GMP synthesis proceeds through two steps, the first being the conversion of IMP to xanthine monophosphate (XMP) catalysed by IMP dehydrogenase followed by GMPS (guanosine 5′-monophosphate synthetase; EC 6.3.5.2) converting XMP to GMP4. GMPS is a class-I (trpG-type) amidotransferase in which the catalytic reaction occurs in two physically distant domains, a GATase (glutamine amidotransferase) domain and an ATPPase (ATP pyrophosphatase) domain5. Hydrolysis of glutamine to glutamate and ammonia occurs in the GATase domain, whereas formation of the intermediate AMP-XMP from ATP and XMP occurs in the ATPPase domain. Ammonia generated in the GATase domain attacks the intermediate to generate GMP.

The glutamine-bound C89A mutant is the first GMPS structure harbouring an original conformation, in which the GATase domain (1–236) has undergone an important reorientation as compared with that seen for the native enzyme. This glutamine-bound structure corresponds to a pre-catalytic state which to the best of our knowledge has never been observed before for this enzyme family. In the structure of PfGMPS_C89A/Gln, glutamine interacts with catalytic site residues Gln93, Asn169, Asn171 and Asp172. This is the first time that a glutamine co-substrate has been observed in a GMPS structure. In this orientation, glutamine is within hydrogen-bonding distance (3.3 Å) of the catalytic residue Cys/Ala89, the ensemble mimicking the pre-catalytic state of the GATase domain. Upon superposition of the PfGMPS- (conformational state I) and PfGMPS_C89A/Gln (conformational state II) dimer structures, the two ATPPase domains remain invariant, whereas the two GATase domains differ by an 85° rotation and a 3 Å translation when going from states I to II. This 85° GATase domain rotation locked by a disulfide bond between Cys113 and Cys377 implies a linker conformational change. Electron density is present for residues 376–389 and 397–401, while in the full-length form and in other reported structures (except HsGMPS) the lid is not visible in the electron density. Transition to conformational state II results in loop 376–401 (lid) being deeply buried into the ATPPase domain. Ultimately, after the conformational change to state II, the helix 371–375 bending would be at a maximum and the lid would be at the bottom of the ATPPase domain, displacing the products of the reaction. This hypothesis is reinforced by Asp371 interacting with Lys386 in PfGMPS_C89A/Gln, thereby blocking the enzyme in an inactive conformation.

> MASHHHHHHGSMAEGEEYDKILVLNFGSQYFHLIVKRLNNIKIFSETKDYGVELKDIKDMNIKGVILSGGPYSVTEAGSPHLKKEVFEYFLEKKIPIFGIAYGMQEIAVQMNGEVKKSKTSEYGCTDVNILRNDNINNITYCRNFGDSSSAMDLYSNYKLMNETCCLFENIKSDITTVWMNHNDEVTKIPENFYLVSSSENCLICSIYNKEYNIYGVQYHPEVYESLDGELMFYNFAYNICKCKKQFDPIRYHELELKNIEKYKHDHYVIAAMSGGIDSTVAAAYTHKIFKERFFGIFIDNGLLRKNEAENVYTFLKSTFPDMNITKIDASENFLSNLQGVTDPEQKRKIIGKLFIEEFEKAVNNIDIDINKTFLLQGTLYPDIIESKCSKNLSDTIKTHHNVGGLPKNLKFKLFEPFKYLFKDDVKTLSRELNLPEEITNRHPFPGPGLAIRVIGEINKHKLNILREVDDIFINDLKQYGLYNQISQAFAVLLSSKSVGVRGDARSYDYVCVLRAVKTSSFMTANWYQIPYDILDKITTRILSEVKGVNRILYDVSSKPPATIEFE>[2x]MHYVTPDLCDAYPELVQVVEPMFSNFGGRDSFGGEIVTIKCFEDNSLVKEQVD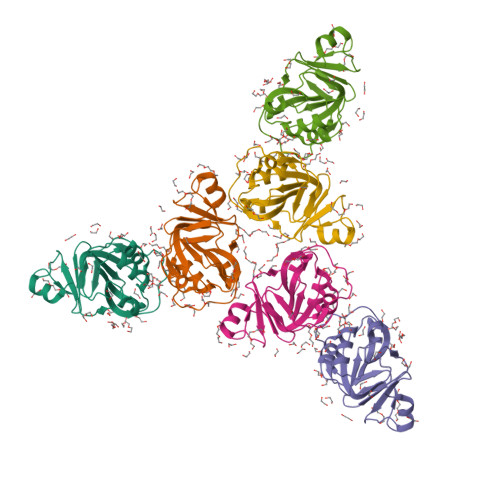KDGKGKVLVVDGGGSLRRALLGDMLAEKAAKNGWEGIVVYGCIRDVDVIAQTDLGVQALASHPLKTDKRGIGDLNVAVTFGGVTFRPGEFVYADNNGIIVSPQALKMPE>AQVQQLTPAQQAALRNQQAMAANLQARQIVLQQSYPVIQQVETQTFDPANRSVFDVTPANVGIVKGFLVKVTAAITNNHATEAVALTDFGPANLVQRVIYYDPDNQRHTETSGWHLHFVNTAKQGAPFLSSMVTDSPIKYGDVMNVIDAPATIAAGATGELTMYYWVPLAYSETDLTGAVLANVPQSKQRLKLEFANNNTAFAAVGANPLEAIYQGAGAADCEFEEISYTVYQSYLDQLPVGQNGYILPLIDLSTLYNLENSAQAGLTPNVDFVVQYANLYRYLSTIAVFDNGGSFNAGTDINYLSQRTANFSDTRKLDPKTWAAQTRRRIATDFPKGVYYCDNRDKPIYTLQY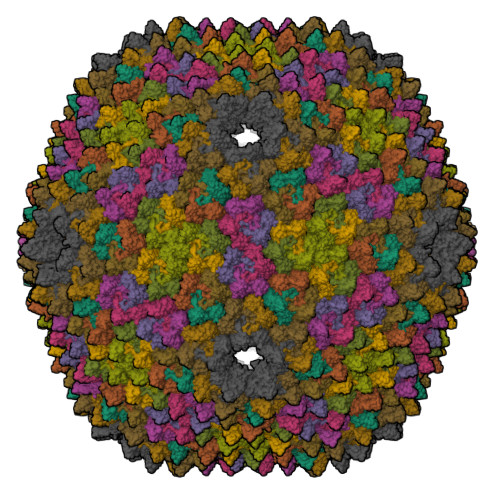GNVGFVVNPKTVNQNARLLMGYEYFTSRTELVNAGTISTT[12x]> XKKRYSREFLLG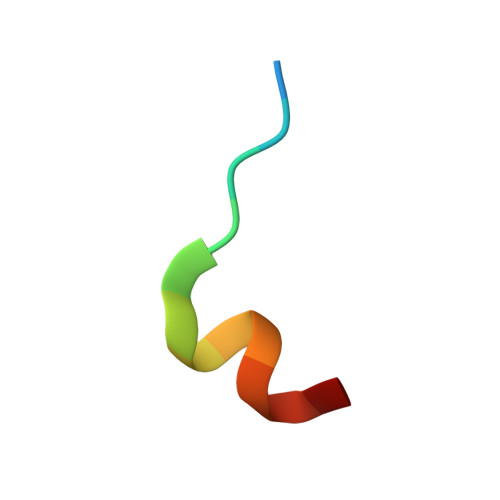FX>SRISPNVYDHSYKRFKSDSLIKRREDITGLRSFVRASLRTPTTVSVSDFGAKGDGKTDDTQAFVNAWKKACSSNGAVNLLVPKGNTYLLKSIQLTGPCNSILTVQIFGTLSASQKRSDYKDISKWIMFDGVNNLSVDGGDTGVVDGNGETWWQNSCKRNKAKPCTKAPTALTFYNSKSLIVKNLKVRNAQQIQISIEKCSNVQVSNVVVTAPADSPNTDGIHITNTQNIRVSESIIGTGDDCISIESGSQNVQINDITCGPGHGISIGSLGDDNSKAFVSGVTVDGAKLSGTDNGVRIKTYQGGSGTASNIIFQNIQMDNVKNP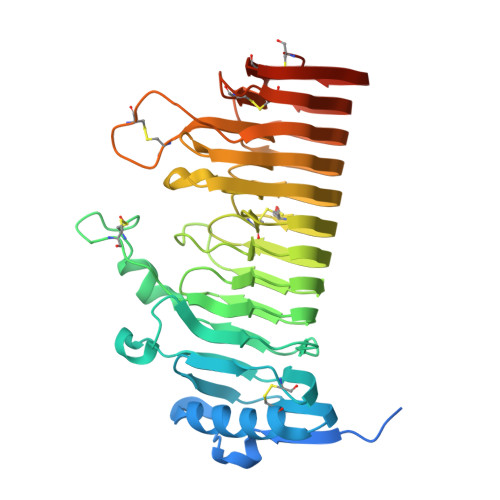IIIDQDYCDKSKCTTEKSAVQVKNVVYRDISGTSASENAITFNCSKNYPCQGIVLDRVNIKGGKATCTNANVVDKGAVLPQCNSTGGRVDHHHHHH[2x]>GSTLKEQIGMRALNVAETVASTSLVREAFRDSNPSVRLQPFAERIRQKTGAEYVVIGNRQGIRYAHPLTERIGKSMIGGDNKEVLKGKSIISEAVGSLGPAIRGKAPIFDENGSVIGIVSVGFLLEDIQRT[8x]

Membrane bound histidine kinases (HKs) are ubiquitous sensors of extracellular stimuli in bacteria. Here, we used solid-state NMR in conjunction with crystallography, solution NMR and distance measurements to investigate the transmembrane signaling mechanism of a paradigmatic citrate sensing membrane embedded HK, CitA. In accordance with the naming of the PASc domain, the periplasmic domain is termed PASp here. The PASp and PASc domains are connected to the TM2 helix by two linkers: the PASp/TM2-linker and the TM2/PASc-linker (topology and domain organization shown in Fig. 1A).

Citrate binding in the sensory extracytoplasmic PAS domain (PASp) causes the linker to transmembrane helix 2 (TM2) to adopt a helical conformation. This triggers a piston-like pulling of TM2 and a quaternary structure rearrangement in the cytosolic PAS domain (PASc). The contraction of the overall β-scaffold of PASp leads to a random coil to α-helix transition in the PASp/TM2-Linker. Based on chemical shift assignment (BMRB ID: 51759 and 51760), we are able to extend this helical characterization to four more amino acids up to I158, which is only one residue away from the predicted membrane embedded region based on cysteine accessibility in the homologous protein DcuS8. This result is in agreement with the conversion of the disordered region downstream of the last β-strand in the PASp core (residues 152-158) in the citrate-free state to a helix (P-helix) extending to the TM2 helix, in the bound state. Structural changes include the P-helix formation, which promotes the piston-like pulling of the TM2 helix, and the amplification of this upward motion by the helical conversion of residues 180GAVG183, which border the membrane and the cytosol. The large change in quaternary structure upon citrate binding detected by CODEX, is represented by the high-resolution structures of PASp and PASc dimers, and together with changes in secondary structure identified by NMR chemical shifts, the mechanism of transmembrane signaling is revealed.> GAMGRRGLVAPQNTFLENIVRRSNDTNFVLGNAQIVDWPIVYSNDGFCKLSGYHRAEVMQKSSACSFMYGELTDKDTVEKVRQTF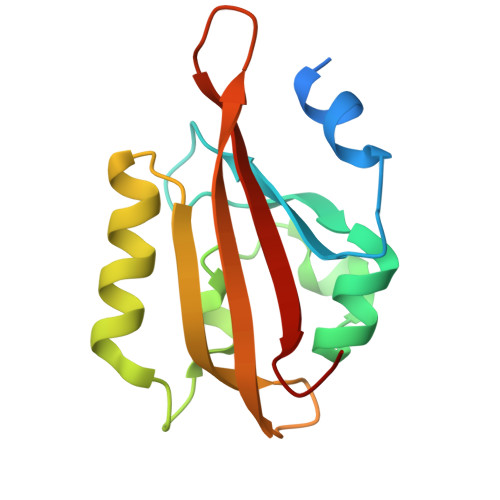ENYEMNSFEILMYKKNRTPVWFFVKIAPIRNEQDKVVLFLCTFSDITAF[(2R)-5-chloro-7-{2-[(2S)-1-chloro-2,3-dihydroxypropan-2-yl]thieno[3,2-b]pyridin-7-yl}-2,3-dihydro-1-benzofuran-2-yl](piperazin-1-yl)methanone | C23 H23 Cl2 N3 O4 S 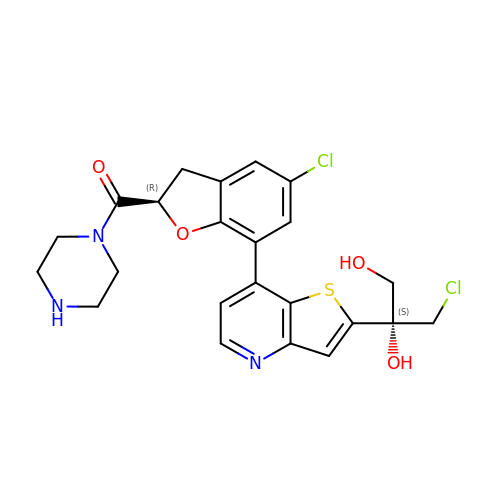| QPYNPPDGRISUAE-JPYJTQIMSA-N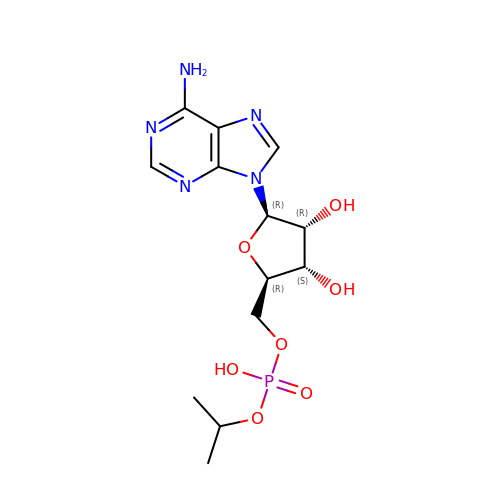5'-O-{(R)-hydroxy[(propan-2-yl)oxy]phosphoryl}adenosine | C13 H20 N5 O7 P | UCVFYZHKFZWYCU-QYVSTXNMSA-N> FNLEHPFFFTNNDYSTDTSIKYQASLPFNWHEVMNNDEWVYQYPIGKFVERQGWKIHISSEYNSSHELLQDVAKICHEMRIPFKHLSTEDKFIMRNGKVVSRGFSGKFITCYPNQNELESVLQRLESALKQYNGPYILSDKRWDEAPIYLRYGVFRPSRDDEKKVAIDELIVGDEVVKDERLPVFKIPKGIVPPDFLNKWLDKKDKKQGDFPFIIDNAIRFSNSGGIYNARLKEDGKKIILKEARPYTGLGFDGTYSSEKLASECKALKILNEWSEAPKIYWHGKIWEHTFLGIEHMKGVPLNRWVTNNFPLYEVVDKTKDYLLRVSKIVEKLIDLTNKFHSENVYHQDLHLGNILVKDEDEISIIDWEQAVFSNDEKVVHKVAAPGFRAWRETLPSEIDWYGIRQIAHYLYMPLVTTSDLTYNYVSQTRIEGKKLFESLGYTREHIDYVESLLSYLDSKCPQIENISRKKVLKPMHEIRTIESEQDIQDFIIKLLRGFTLTYGQWRKEFQSRFFPVAYYGLNFNQGIAFSDLAILWSYQQLAKKVKNFKFDDYYEIRTQVINEAVNNFKKSSLSGLFDGKIGTIWLIYEFGEIDRAVELFTTHFIEIFENSQ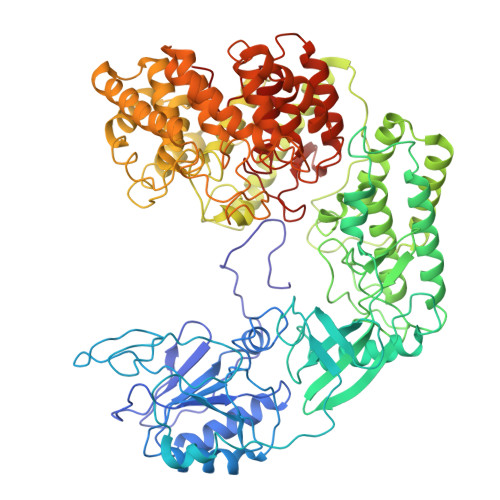NKNLYSGQAGILLVGLYFLSKGEIDNKLGEEILIRLREYTLNYIENPETFCKVGASDVQSNDPYENFGGLLYGHAGVAWLFGEAYKLTGESIYKNGLELAVDKELVAYKVDSNNSLQYSQGHRLLPYLATGSAGLLLLINRNKEILSSKYLKYLTSLERATDVVFCVLPGLFNGFCGLEVANNIYSDIDDNFSGQKKLIEQLYRYLCVIEEGFVIAGDNGLKITTDIASGFAGVAIGLVSIMDNKLTILPQI Class I histone deacetylases (HDACs 1–3) are essential regulators of gene expression. The enzymes are recruited to chromatin as part of large multi-protein complexes that control the acetylation state of histones and other chromatin-associated factors. In the MiDAC complex, the large ELM2-SANT protein MIDEAS (1045 aa), recruits HDAC1 or 2. In conclusion, our structural and functional studies of the MiDAC complex reveal a striking molecular machine whose architecture appears to have evolved to facilitate processive chromatin deacetylation.

In all, 126,484 particles were included in the final ~4-Å map of the dimeric complex with C2 symmetry applied. The structure of the dimeric complex has an overall S shape. It reveals that the ELM2 domain from MIDEAS does not mediate dimerisation. Instead, the MIDEAS ELM2 domain interacts with the DNTTIP1 dimerisation domain which mediates the dimeric assembly. The consequence of this is that the HDAC1 catalytic subunits are arranged very differently, located much farther apart, with the HDAC1 active sites on opposite ends of the dimer. This is a complete contrast with the NuRD complex in which MTA1 dimerisation results in the HDAC1 active sites being positioned on the same face of the complex. The shorter helix in MIDEAS mediates a tight interaction with a non-polar groove between the end of the long helices of the DNTTIP1 dimer. One of the regions of MIDEAS most similar to other ELM2-SANT domain co-repressor proteins is the ELM2-specific motif which binds in an extended conformation in a conserved groove on HDAC1. Density for the InsP6, but not the SAHA, was clearly visible in the map. The dimerisation domain of DNTTIP1 is critical for the assembly of the complex since it interacts with the ELM2 domain of MIDEAS and dictates the relative positioning of the HDACs in the dimer.

>[2x]MGATGDAEQPRGPSGAERGGLELGDAGAAGQLVLTNPWNIMIKHRQVQRRGRRSQMTTSFTDPAISMDLLRAVLQPSINEEIQTVFNKYMKFFQKAALNVRDNVGEEVDAEQLIQEACRSCLEQAKLLFS;>[2x]MAQTQGTRRKVCYYYDGDVGNYYYGQGHPMKPHRIRMTHNLLLNYGLYRKMEIYRPHKANAEEMTKYHSDDYIKFLRSIRPDNMSEYSKQMQRFNVGEDCPVFDGLFEFCQLSTGGSVASAVKLNKQQTDIAVNWAGGLHHAKKSEASGFCYVNDIVLAILELLKYHQRVLYIDIDIHHGDGVEEAFYTTDRVMTVSFHKYGEYFPGTGDLRDIGAGKGKYYAVNYPLRDGIDDESYEAIFKPVMSKVMEMFQPSAVVLQCGSDSLSGDRLGCFNLTIKGHAKCVEFVKSFNLPMLMLGGGGYTIRNVARCWTYETAVALDTEIPNELPYNDYFEYFGPDFKLHISPSNMTNQNTNEYLEKIKQRLFENLRMLPHAPGVQMQAIPEDAIPEESGDEDEDDPDKRISICSSDKRIACEEEFSDSEEEGEGGRKNSSNFKKAKRVKTEDEKEKDPEEKKEVTEEEKTKEEKPEAKGVKEEVKLA;>GAVSIEPRINVGSRFQAEIPLMRDRALAAADPHKADLVWQPWEDLESSREKQRQVEDLLTAACSSIFPGAGTNQELALHCLHESRGDILETLNKLLLKKPLRPHNHPLATYHYTGSDQWKMAERKLFNKGIAIYKKDFFLVQKLIQTKTVAQCVEFYYTYKKQVKIGRNGTLT[2x]>[6x]M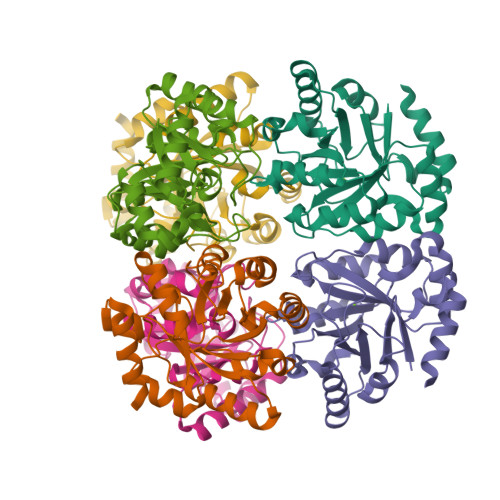KISPSLMCMDLLKFKEQIEFIDSHADYFHIDIMDGHFVPNLTLSPFFVSQVKKLATKPLDCHLMVTRPQDYIAQLARAGADFITLHPETINGQAFRLIDEIRRHDMKVGLILNPETPVEAMKYYIHKADKITVMTVDPGFAGQPFIPEMLDKLAELKAWREREGLEYEIEVDGSCNQATYEKLMAAGADVFIVGTSGLFNHAENIDEAWRIMTAQILAAKSEVQPHAKTA> SMSGIALSRLAQERKAWRKDHPFGFVAVPTKNPDGTMNLMNWECAIPGKKGTPWEGGLFKLRMLFKDDYP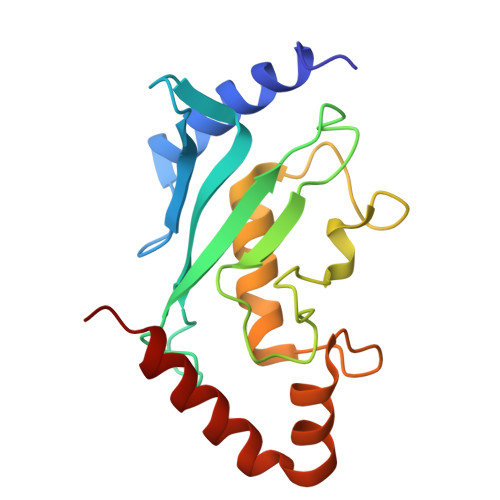SSPPKCKFEPPLFHPNVYPSGTVCLSILEEDKDWRPAITIKQILLGIQELLNEPNIQDPAQAEAYTIYCQNRVEYEKRVRAQAKKFAPS> NKRAPYWTNTEKMEKRLHAVPAANTVKFRCPAGGNPMPTMRWLKNGKEFKQEHRIGGYKVRNQHWSLIMESVVPSDKGNYTCV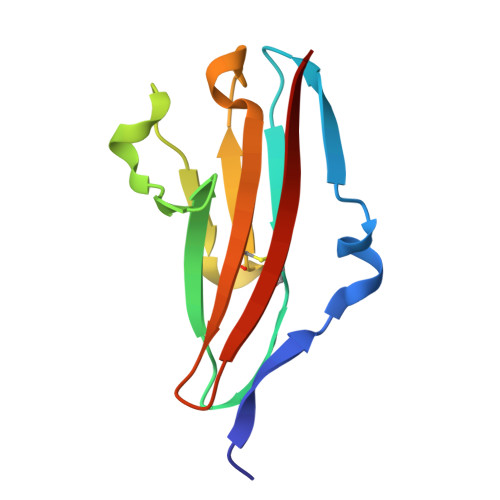VENEYGSINHTYHLDVV N-{4-[(3-chloro-4-fluorophenyl)amino]-7-[(3S)-tetrahydrofuran-3-yloxy]quinazolin-6-yl}-4-(dimethylamino)butanamide | C24 H27 Cl F N5 O3 | 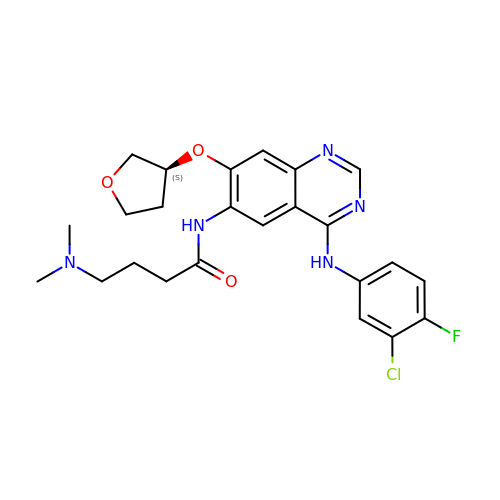JSENTLOBWVHLNR-INIZCTEOSA-N Proteins that perform these functions include Vipp1/IM30 in photosynthetic plastids, PspA in bacteria, and ESCRT-III in eukaryotes. Here, using a combination of evolutionary and structural analyses, we show that these protein families are homologous and share a common ancient evolutionary origin that likely predates the last universal common ancestor. This homology is evident in cryo-electron microscopy structures of Vipp1 rings from the cyanobacterium Nostoc punctiforme presented over a range of symmetries. Rings have an inner lumen that is able to bind and deform membranes.

By reconstructing the C14 symmetry ring (Vipp1C14), we achieved an overall resolution of 6.5 Å with highest resolution regions reaching 4.8 Å. This was sufficient to allow unambiguous assignment of the helical domains within the Vipp1 monomer and asymmetric unit and consequently the entire 2.4 MDa Vipp1C14 ring containing 84 subunits (STAR Methods). To build the Vipp1C14 monomer, a homology model was initially generated from the PspA crystal structure hairpin motif (aa 24–142). The Vipp1 hairpin homology model with its distinct axial twist closely fitted the Vipp1C14 map and acted as an anchor from which to build the remaining main chain. Vipp1C14 rings are assembled from six rungs stacked on top of each other. Each rung differs in conformation so that an asymmetric dome-shaped curvature is achieved when rings are viewed from the side. Rungs are maximally constricted at the top and bottom with internal lumen diameters of 14 nm and 15.7 nm, and widest at the ring equator between rungs 3 and 4 with an internal diameter of 17.5 nm. The basic building block (or asymmetric unit) of Vipp1C14 is a stack of six monomers, each one located in a different rung, which when repeated forms a ring. Intriguingly, the six subunits within each asymmetric unit have distinct conformations, which is made possible by three hinge regions that provide Vipp1 with conformational versatility. As dome-shaped curvature increases toward the top of the ring, helix α5 rotates from being oriented at 40° relative to the horizontal in rung 5 to a maximum of 80° in rung 2.

>[84x]MGLFDRIKRVVSSNLNDLVNKAEDPEKMLEQAILEMQEDLVQLRQGVAQAIAAQKRSEKQYNDAQNEINKWQRNAQLALQKGDENLARQALERKKTYTDTSAALKASLDTQSTQVETLKRNLIQLESKISEAKTKKEMLKARITTAKAQEQLQGMVRGMNTSSAMSAFERMEEKVLMQESRAQALGELAGADLETQFAQLEGGSDVDDELAALKAQMLPPATPVTQAQLPPQQETTPAKSNEVVDAELDSLRKQLDQL>DAAQPARRAVRSSRHHHHHHGSPVCAAPMVFFDCRNATPGDTGAGCQKSCHTLDMTCYSPQCVPGCVCPDGLVADGEGGCITAEDCPCVHNEASYRAGQTIRVGCNTCTCDSRMWRCTDDPCLATCAVYGDGHYLTFDGQSYSFNGDCEYTLVQNHCGGKDSTQDSFRVVTENVPCGTTGTTCSKAIKIFLGGFELKLSHGKVEVIGTDESQEVPYTIRQMGIYLVVDTDIGLVLLWDKKTSIFINLSPEFKGRVCGLCGNFDDIAVNDFATRSRSVVGDVLEFGNSWKLSPSCPDALAPKDPCTANPFRKSWAQKQCSILHGPTFAACHAHVEPARYYEACVNDACACDSGGDCECFCTAVAAYAQACHEVGLCVSWRTPSICPLFCDYYNPEGQCEWHYQPCGVPCLRTCRNPRGDCLRDVRGLEGCYPKCPPEAPIFDEDKMQCVATCPTPPLPPRCHVHGKSYRPGAVVPSDKNCQSCLCTERGVECTYKAEACVCTYNGQRFHPGDVIYHTTDGTGGCISARCGANGTIERRVYPCSPTTPVPPTTFSFSTPPLVVSSTHTPSNGPSSAHTGPPSSAWPTTAGTSPRTRLPTASASLPPVCGEKCLWSPWMDVSRPGRGTDSGDFDTLENLRAHGYRVCESPRSVECRAEDAPGVPLRALGQRVQCSPDVGLTCRNREQASGLCYNYQIRVQCCTPLPCTSEQKLISEEDLSRKLTR[2x]

The two gel-forming mucins MUC5AC and MUC5B constitute the main structural components of the mucus protecting the underlying epithelia in the respiratory system. The VWD assemblies are formed by the VWD domain, C8, trypsin inhibitor like (TIL) and E domains, except the VWD’ domain that only has the TIL and E domains. We determined the cryoEM structures of the wild type D3 assembly of the human MUC5AC mucin and the structural single nucleotide polymorphisms (SNP) variants Arg996Gln and Arg1201Trp that affect intermolecular interactions. The D3 assembly forms covalent dimers that can appear in two alternative conformations, open and closed, where the closed conformation dimers interact through an arginine-rich loop in the TIL3 domain to form tetramers.

The structure of the MUC5AC-D3 assembly was analyzed by cryoEM at pH 7.4. The cryoEM reconstruction of the D’-D3-CysD1 recombinant protein reached higher resolution (3.2 Å) than the isolated D3, even if only the D3 assembly is visible due to flexibility of the D’ and CysD1 domains. The covalent MUC5AC-D3 assembly dimer is formed via two intermolecular disulfide bonds, Cys1132-Cys1132 in the C8-3 domain and Cys1174-Cys1174 in the TIL3 domain. However, the Cys1132 intermolecular disulfide bond is partially reduced as observed previously in MUC2-D3. The MUC5AC-TIL3 β1-β2 loop, unlike the other mucins and VWF, is remarkably rich in arginines (20%). In MUC2 and VWF, the center of the TIL3 β1-β2 loop is located only 6.2 Å and 8.8 Å away from VWD3 β9, while in MUC5AC they are separated by 14.4 Å. During the 3D-classification processes, a second MUC5AC-D3 assembly conformation was observed. These were estimated to represent 17% of the total MUC5AC particles. Here the first mucin D3 assembly solved at neutral pH is presented. Interestingly no major structural differences were observed compared to the low pH.> SLDVLIVYELTPTAEQKALATKLKLPPTFFCYKN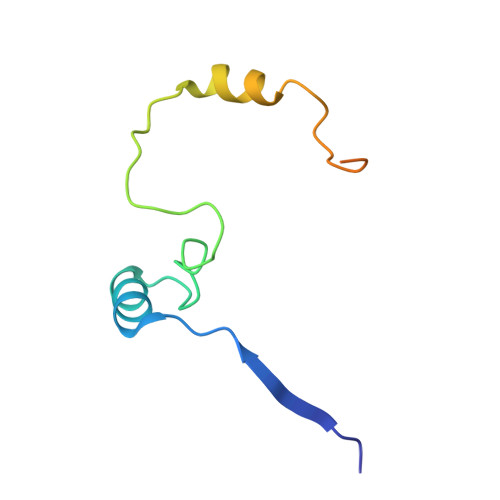RPDYVSEEEEDDEDFETAVKKLNGKLYLDGSEKCRPLEENTADNEKECI>[3x]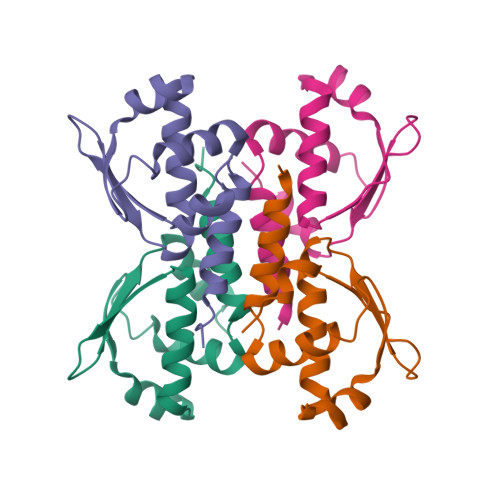GSSHHHHHHMSKAVVQMAISSLSYSELEAIEHIFEELDGNEGLLVASKIADRVGITRSVIVNALRKLESAGVIESRSLGMKGTYIKVLNNKFLIELENLKSH> MVSTLKPLKIGKHTIKFPIFQGGMGVGISWDELAGNVAKEGALGVISAVGTGYYKNMRFVERIVAKKPFEALNFYSKKALNEIFANARKICGNNPLG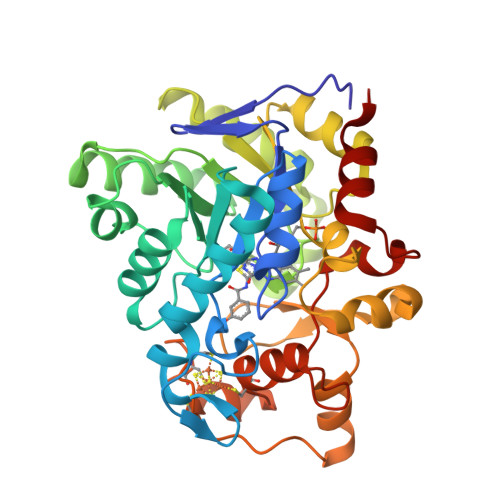ANILYAINDYGRVLRDSCEAGANIIITGAGLPTNMPEFAKDFSDVALIPIISSAKALKILCKRWSDRYKRIPDAFIVEGPLSGGHQGFKYEDCFKEEFRLENLVPKVVEASKEWGNIPIIAAGGIWDRKDIDTMLSLGASGVQMATRFLGTKECDAKVYADLLPTLKKEDILLIKSPVGYPARAINTGVIKRIEEGNAPKIACVSNCVAPCNRGEEAKKVGYCIADGLGRSYLGNREEGLYFTGANGYRVDKIISVHELIKELTEG> GAMTFTRYSRLRVIAEIRHGDIFHSANIVSSIEFDRDDELFATAGVSRCIKVFDFSSVVNEPADMQCPIVEMSTRSKLSCLSWNKHEKNHIASSDYEGIVTVWDVTTRQSLMEYEEHEKRAWSVDFSRTEPSMLVSGSDDCKVKVWCTRQEASVINIDMKANICCVKYNPGSSNYIAVGSADHHIHYYDLRNISQPLHVFSGHKKAVSYVKFLSNNELASASTDSTLRLWDVKDNLPVRTFRGHTNEKNFVGLTVNSEYLACGSETNEVYVYHKEITRPVTSHRFGSPDMDDAEEEAGSYFISAVCWKSDSPTMLTANSQGTIKVLVLAA;> XEHFIVPDLY

The COP1 E3 ubiquitin ligase is a central signaling hub that integrates inputs from plant light‐sensing photoreceptors. COP1 contains an N‐terminal zinc finger, a central coiled‐coil, and a C‐terminal WD40 domain, which is essential for proper COP1 function (Deng et al, 1992; McNellis et al, 1994). COP1 regulates gene expression and plays a central role as a repressor of photomorphogenesis by directly modulating the stability of transcription factors that control the expression of light‐regulated genes.

Next, we obtained crystal structures for the different peptides bound to COP1 (1.3–2.0 Å resolution, see Tables EV1 and EV2, and EV4) to compare their peptide binding modes. We found that all peptides bind in a similar configuration with the VP forming the center of the binding site (r.m.s.d. between the different peptides range from ~ 0.3 to 1.5 Å, comparing 5 or 6 corresponding Cα atoms). Chemically diverse amino acids (Tyr/Arg/Gln) map to the −3 and −2 position and often deeply insert into the COP1 binding cleft, acting as anchor residues. This suggests that the COP1 WD40 domain has high structural plasticity, being able to accommodate sequence‐divergent VP‐containing peptides. C Superposition of the VP peptide binding modes of the HY5 (green), COL3 (orange), and STO (gray) peptides depicted in ball‐and‐stick representation when bound to the COP1 WD40 domain as observed in their respective X‐ray crystal structures.>[2x]GSHMASMTGGQQMGRGSMQQQDFPAGTTPNEHNINGADYPRIGEDRRVHFRIHAPNAQKVEISFRGEMTKEADGYWSLVSKEPEVIGFHYYQVIIDGVSAADPNGKPFFGMGKWVSGIEIPEKGVDYYSIKNVPHGLISQSWYYSDIRKEWRRCIVYTPAEYDKNPTKKYPVLYLQHGMGENET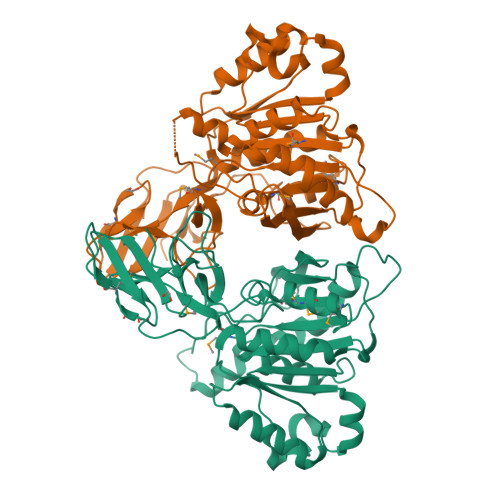SWANQGKMNFIMDNLIAEGKAKPMIVVMDNGNIEVFKTNSGETPEDARKRFGAEFPAILVNEIIPHIESNFRTLTDRDNRAMAGLSWGGLLTFNTTLNNLDKFAYIGGFSGAGSIDLKQLDTVYGGVFKNRKAFNDKVHVFFLGIGSEEHPERTKNLSDGLQAAGINTIYYESPGTAHEFLTWRRCLKEFAPLLFKTK>[2x]GSHMAGAQDFVPHTADLAELAAAAGE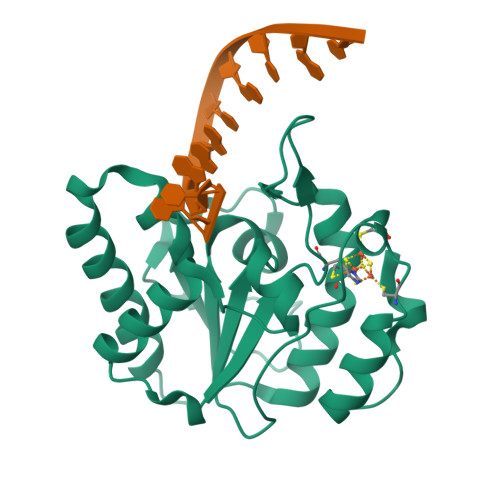CRGCGLYRDATQAVFGAGGRSARIMMIGEQPGDKEDLAGLPFVGPAGRLLDRALEAADIDRDALYVTNAVKHFKFTRAAGGKRRIEKTPSRTEVVACRPWLIAEMTSVEPDVVVLLGATAAKALLGNDFRVTQHRGEVLHVDDVPGDPALVATVHPSSLLRGPKEERESAFAGLVDDLRVAADVRP> MSKKRVVKLRELVPAVAALAVAVLIQSATGSSGGSGHTPTTQATHADDHDLTTHNGTEEHDDGHDDGHDDLHAHAPKVIVFISGSCLFGAISRSLFKKLPIPYTVVLLILGAILGVVASNVPLVEEHTRDVAHMDPHVLLQIFLPVLIFESAFAMDVHTFMRSFSQVCILALFGLVVASVLTAVLAMNLFNYNWNFSEAMMFGAIMSATDPVAVVALLKDLGASKQLGTIIEGESLLNDGCAIVIFNVFMKMVFFPQLTSTVGQNVLYFLQVAVAGPLWGYAVAKVTVFFLSHIFNDALVEITITLAATYLTYYIGDIWLEVSGVLAVVVLGLIVNAEKTSISPEVEVFLHRFWEMLAYLANTLIFMMVGVVVTQKALVAVDKMDWFYLIILYLAITIIRGMVISLFSPILSRIGYGLTWRNAVIMTWGGLRGAVGLALALVVENLAGNDVIGSKFLFHTAGIVVLTLVINATTIQTLLRILGMSDISIPKRLAMAGAVRRIHEGQNRTLNMLKSDRFLADADWDIATAACEISDPYSALSDDENAPADELTLGERKSVCPGCKAMVPNEPSPREFADMMEEARLRMLKAEKISYWKQFEHGMLAREALRLLVQHAEVAADEKDQFILVDDLKKSWQIKGIYPWLKRKLEDLISEKKIAAIPMPKYKLGKLMYKICHHMAFEVTINIAIVLNIVPIIMEFVVQDKMASVSTMAAPGSTVSSEPSSSQKIEDALRISNYVFFVIYAIEAIVKILGLGRHYIVSHWNKFDAFILVVALVDIIIAETLLKGSITINLSSIKVVKLFRLLRGLRMLRLTKALIPKLILVVNGKINNQLSLGYDVGKGYIIGEEEVGKIIDRMVDNKKILRELKHISET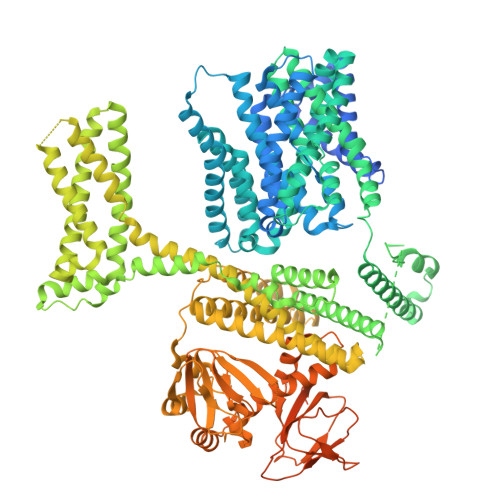GRLQVVKELGLLQREHPGIAVSVKTRQAIRTILNHSRETIHELQGAGLLDEMEAHKLELTVEIKMKRLMNAPSSIPPPPPENLLKNVSWLAGDMKLIDFIKARASLLHFDYGEVIVREGDESDGLFLIVSGLVKLYGKSAFLDHDNPPVTAGSEENEVFEDYLTVGNVIGEMGVLTKKPRNATVTCETTVQVYFITAEDMNIAIDTFTLYPSLEYRLWRVVAIRIATPLIMEQMAFQGWTQEKVKLHLERGYLVDLAESHFQFNIDATLEDVILINGTAYNAHTREEIRSPCLISRTVHKLTFQYTATEEPRLFVVRNAEYNGPILDGRLDVDSKRSLISITEISSNMCLKHAAELRQKNSKVMLSRKSSGAAAKEEEDCIPNTSDVEQAAGVSPSVPTKTTPKPKSFLPSLGLSMSKERVNGEAVEESPVKTKQGEETPETEEGAAPRVNVALEVLFQ>[4x]AECSVDIQGNDQMQFNTNAITVDKSCKQFTVNLSHPGNLPKNVMGHNFVLSTAADMQGVVTDGMASGLDKDFLKPDDSRVIAQTKLIGSGEKDSVTFDVSKLKEGEQFMFFCTFPGH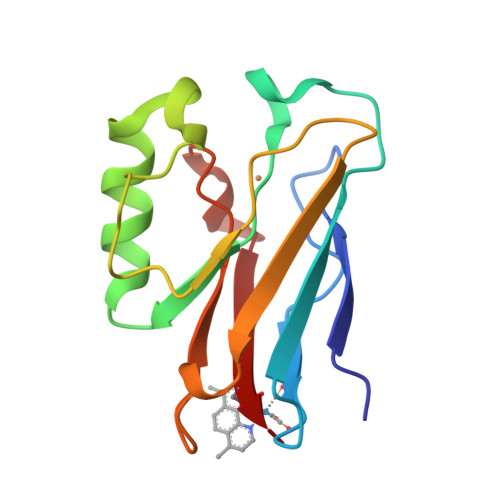SALMWGWLHLK>[6x]SMGFWEASSRGGGAFSGGEDASEGGAEEGAGGAGGSAGAGEGPVITALTPMTIPDVFPHLPLIAITRNPVFPRFIKIIEVKNKKLVELLRRKVRLAQPYVGVFLKRDDSNESDVVESLDEIYHTGTFAQIHEMQDLGDKLRMIVMGHRRVHISRQLEVEPEEPEAENKHKPRRKSKRGKKEAEDELSARHPAELAMEPTPELPAEVLMVEVENVVHEDFQVTEEVKALTAEIVKTIRDIIALNPLYRESVLQMMQAGQRVVDNPIYLSDMGAALTGAESHELQDVLEETNIPKRLYKALSLLKKEFELSKLQQ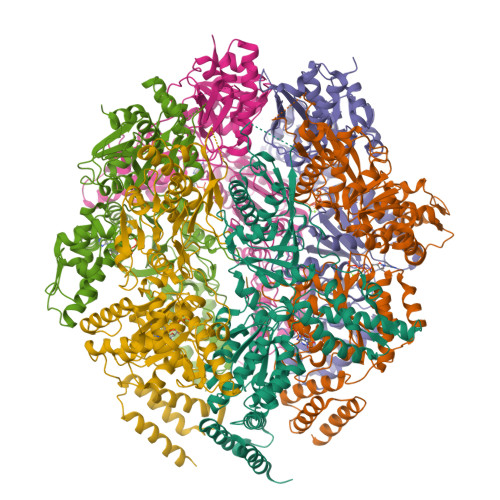RLGREVEEKIKQTHRKYLLQEQLKIIKKELGLEKDDKDAIEEKFRERLKELVVPKHVMDVVDEELSKLGLLDNHSSEFNVTRNYLDWLTSIPWGKYSNENLDLARAQAVLEEDHYGMEDVKKRILEFIAVSQLRGSTQGKILCFYGPPGVGKTSIARSIARALNREYFRFSVGGMTDVAEIKGHRRTYVGAMPGKIIQCLKKTKTENPLILIDEVDKIGRGYQGDPSSALLELLDPEQNANFLDHYLDVPVDLSKVLFICTANVTDTIPEPLRDRMEMINVSGYVAQEKLAIAERYLVPQARALCGLDESKAKLSSDVLTLLIKQYCRESGVRNLQKQVEKVLRKSAYKIVSGEAESVEVTPENLQDFVGKPVFTVERMYDVTPPGVVMGLAWTAMGGSTLFVETSLRRPQDKDAKGDKDGSLEVTGQLGEVMKESARIAYTFARAFLMQHAPANDYLVTSHIHLHVPEGATPKDGPSAGCTIVTALLSLAMGRPVRQNLAMTGEVSLTGKILPVGGIKEKTIAAKRAGVTCIVLPAENKKDFYDLAAFITEGLEVHFVEHYREIFDIAFPD> MAAHRPVEWVQAVVSRFDEQLPIKTGQQNTHTKVSTEHNKECLINISKYKFSLVISGLTTILKNVNNMRIFGEAAEKNLYLSQLIILDTLEKCLAGQPKDTMRLDETMLVKQLLPEICHFLHTCREGNQHAAELRNSASGVLFSLSCNNFNAVFSRISTRLQELTVCSEDNVDVHDIELLQYINVDCAKLKRLLKETAFKFKALKKVAQLAVINSLEKAFWNWVENYPDEFTKLYQIPQTDMAECAEKLFDLVDGFAESTKRKAAVWPLQIILLILCPEIIQDISKDVVDENNMNKKLFLDSLRKALAGHGGSRQLTESAAIACVKLCKASTYINWEDNSVIFLLVQSMVVDLKNLLFNPSKPFSRGSQPADVDLMIDCLVSCFRISPHNNQHFKICLAQNSPSTFHYVLVNSLHRIITNSALDWWPKIDAVYCHSVELRNMFGETLHKAVQGCGAHPAIRMAPSLTFKEKVTSLKFKEKPTDLETRSYKYLLLSMVKLIHADPKLLLCNPRKQGPETQGSTAELITGLVQLVPQSHMPEIAQEAMEALLVLHQLDSIDLWNPDAPVETFWEISSQMLFYICKKLTSHQMLSSTEILKWLREILICRNKFLLKNKQADRSSCHFLLFYGVGCDIPSSGNTSQMSMDHEELLRTPGASLRKGKGNSSMDSAAGCSGTPPICRQAQTKLEVALYMFLWNPDTEAVLVAMSCFRHLCEEADIRCGVDEVSVHNLLPNYNTFMEFASVSNMMSTGRAALQKRVMALLRRIEHPTAGNTEAWEDTHAKWEQATKLILNYPKAKMEDGQAAESLHKTIVKRRMSHVSGGGSIDLSDTDSLQEWINMTGFLCALGGVCLQQRSNSGLATYSPPMGPVSERKGSMISVMSSEGNADTPVSKFMDRLLSLMVCNHEKVGLQIRTNVKDLVGLELSPALYPMLFNKLKNTISKFFDSQGQVLLTDTNTQFVEQTIAIMKNLLDNHTEGSSEHLGQASIETMMLNLVRYVRVLGNMVHAIQIKTKLCQLVEVMMARRDDLSFCQEMKFRNKMVEYLTDWVMGTSNQAADDDVKCLTRDLDQASMEAVVSLLAGLPLQPEEGDGVELMEAKSQLFLKYFTLFMNLLNDCSEVEDESAQTGGRKRGMSRRLASLRHCTVLAMSNLLNANVDSGLMHSIGLGYHKDLQTRATFMEVLTKILQQGTEFDTLAETVLADRFERLVELVTMMGDQGELPIAMALANVVPCSQWDELARVLVTLFDSRHLLYQLLWNMFSKEVELADSMQTLFRGNSLASKIMTFCFKVYGATYLQKLLDPLLRIVITSSDWQHVSFEVDPTRLEPSESLEENQRNLLQMTEKFFHAIISSSSEFPPQLRSVCHCLYQVVSQRFPQNSIGAVGSAMFLRFINPAIVSPYEAGILDKKPPPRIERGLKLMSKILQSIANHVLFTKEEHMRPFNDFVKSNFDAARRFFLDIASDCPTSDAVNHSLSFISDGNVLALHRLLWNNQEKIGQYLSSNRDHKAVGRRPFDKMATLLAYLGPPEHKPVADTHWSSLNLTSSKFEEFMTRHQVHEKEEFKALKTLSIFYQAGTSKAGNPIFYYVARRFKTGQINGDLLIYHVLLTLKPYYAKPYEIVVDLTHTGPSNRFKTDFLSKWFVVFPGFAYDNVSAVYIYNCNSWVREYTKYHERLLTGLKGSKRLVFIDCPGKLAEHIEHEQQKLPAATLALEEDLKVFHNALKLAHKDTKVSIKVGSTAVQVTSAERTKVLGQSVFLNDIYYASEIEEICLVDENQFTLTIANQGTPLTFMHQECEAIVQSIIHIRTRWELSQPDSIPQHTKIRPKDVPGTLLNIALLNLGSSDPSLRSAAYNLLCALTCTFNLKIEGQLLETSGLCIPANNTLFIVSISKTLAANEPHLTLEFLEECISGFSKSSIELKHLCLEYMTPWLSNLVRFCKHNDDAKRQRVTAILDKLITMTINEKQMYPSIQAKIWGSLGQITDLLDVVLDSFIKTSATGGLGSIKAEVMADTAVALASGNVKLVSSKVIGRMCKIIDKTCLSPTPTLEQHLMWDDIAILARYMLMLSFNNSLDVAAHLPYLFHVVTFLVATGPLSLRASTHGLVINIIHSLCTCSQLHFSEETKQVLRLSLTEFSLPKFYLLFGISKVKSAAVIAFRSSYRDRSFSPGSYERETFALTSLETVTEALLEIMEACMRDIPTCKWLDQWTELAQRFAFQYNPSLQPRALVVFGCISKRVSHGQIKQIIRILSKALESCLKGPDTYNSQVLIEATVIALTKLQPLLNKDSPLHKALFWVAVAVLQLDEVNLYSAGTALLEQNLHTLDSLRIFNDKSPEEVFMAIRNPLEWHCKQMDHFVGLNFNSNFNFALVGHLLKGYRHPSPAIVARTVRILHTLLTLVNKHRNCDKFEVNTQSVAYLAALLTVSEEVRSRCSLKHRKSLLLTDISMENVPMDTYPIHHGDPSYRTLKETQPWSSPKGSEGYLAATYPTVGQTSPRARKSMSLDMGQPSQANTKKLLGTRKSFDHLISDTKAPKRQEMESGITTPPKMRRVAETDYEMETQRISSSQQHPHLRKVSVSESNVLLDEEVLTDPKIQALLLTVLATLVKYTTDEFDQRILYEYLAEASVVFPKVFPVVHNLLDSKINTLLSLCQDPNLLNPIHGIVQSVVYHEESPPQYQTSYLQSFGFNGLWRFAGPFSKQTQIPDYAELIVKFLDALIDTYLPGIDEETSEESLLTPTSPYPPALQSQLSITANLNLSNSMTSL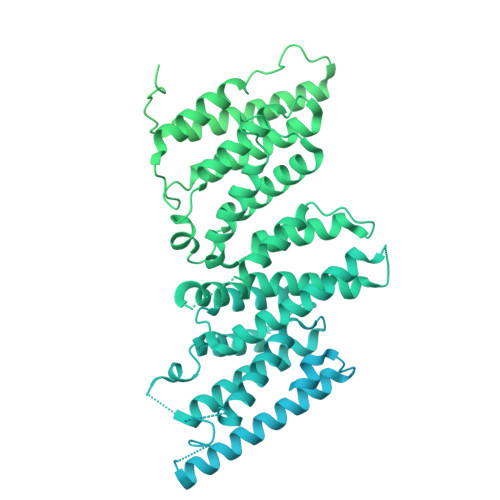ATSQHSPGIDKENVELSPTTGHCNSGRTRHGSASQVQKQRSAGSFKRNSIKKIV> MGVEKVPKYDIPTKKVDYVFIELDKMKPHAQLVQKELEAFIESVTGSGIFWKPMLLAKVPGE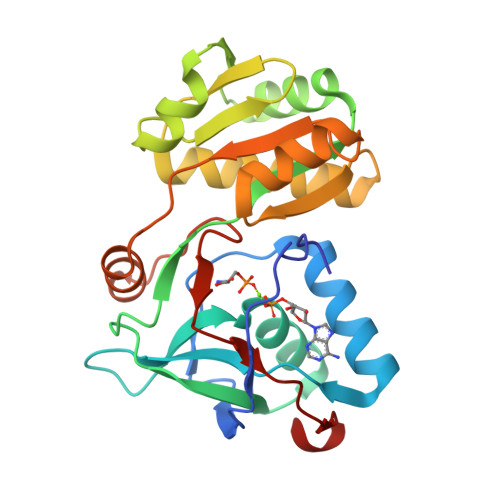DMYLIVDGHHRWAGLQKLGAKRAPSVILDYFSDDVKVYTWYPAFKGDLNEVVERLKKEGLEVIEDPEAEEKAERGEIAFALVGEKSFAIPGGLEEQKKVSKVLDEMSVEGKIELIYYGLKEDAREDMAKGEIDYVFIRKAPTKEEVMELVKRGEVYSPKTTRHVLPFNPDKIDVKLEELF>GPGSEFKSMTQEAFQESSVKELGRLEAQLASLRQELAALTLKQNSVADEVGL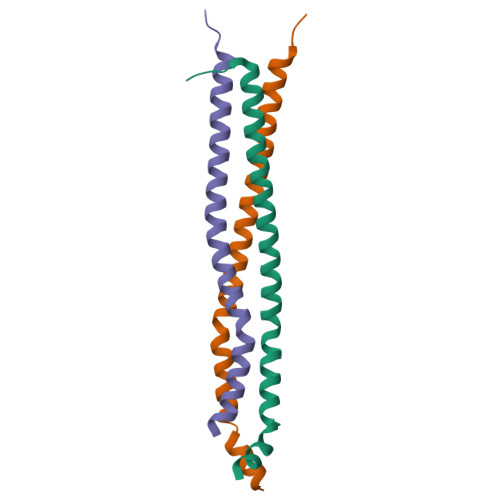LPQKIQAARADVESQFPDWIRQFLLG[3x]>[2x]GPGGGGSVTCPGGQSTSNSQCCVWFDVLDDLQTNFYQGSKCESPVRKILRIVFHDAIGF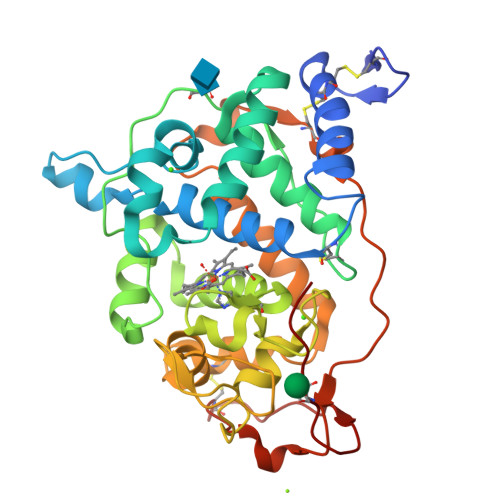SPALTAAGQFGGGGADGSIIAHSNIELAFPANGGLTDTVEALRAVGINHGVSFGDLIQFATAVGMSNCPGSPRLEFLTGRSNSSQPSPPSLIPGPGNTVTAILDRMGDAGFSPDEVVDLLAAHSLASQEGLNSAIFRSPLDSTPQVFDTQFYIETLLKGTTQPGPSLGFAEELSPFPGEFRMRSDALLARDSRTACRWQSMTSSNEVMGQRYRAAMAKMSVLGFDRNALTDCSDVIPSAVSNNAAPVIPGGLTVDDIEVSCPSEPFPEIATASGPLPSLAPAP>TPEMPVLENRAAQGDITAPGGARRLTGDQTAALRDSLSDKPAKNIILLIGDGMGDSEITAARNYAEGAGGFFKGIDALPLTGQYTHYALNKKTGKPDYVTDTAASATAWSTGVKTYNGALGVDIHEKDHPTILEMAKAAGLATGNVSTAELQDATPAALVAHVTSRKCYGPSATSEKCPGNALEKGGKGSITEQLLNARADVTLGGGAKTFAETATAGEWQGKTLREQAQARGYQLVSDAASLNSVTEANQQKPLLGLFADGNMPVRWLGPKATYHGNIDKPAVTCTPNPQRNDSVPTLAQMTDKAIELLSKNEKGFFLQVEGASIDKQDHAANPCGQIGETVDLDEAVQRALEFAKKEGNTLVIVTADHAHASQIVAPDTKAPGLTQALNTKDGAVMVMSYGNSEEDSQEHTG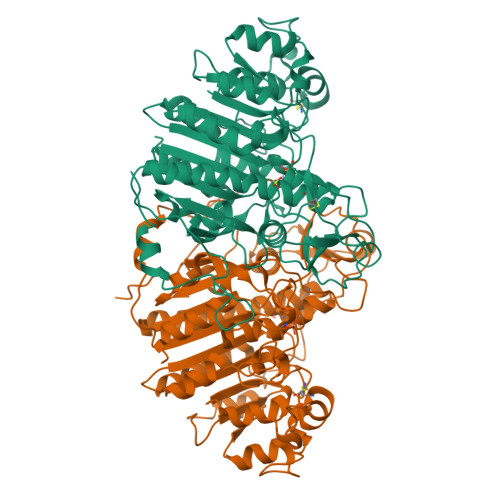SQLRIAAYGPHAANVVGLTDQTDLFYTMKAALGLK[2x]As the virus buds from the cell, the viral protease cleaves Gag into several fragments, including the capsid protein (CA) that then assembles into the mature capsid shell (core), rendering the virus particle infectious. The CA portion of all retroviral Gag proteins folds into two separate domains, the N-terminal domain (CANTD) and C-terminal domain (CACTD). In mature lattices, CANTD interactions form only intra-hexamer and intra-pentamer interfaces, while CACTD interactions are also involved in formation of inter-hexamer and inter-pentamer interfaces. Our results show that, like lentiviruses, RSV is sensitive to IP6 in vitro and in cells, where in the mature CA lattice IP6 binds in a pore formed in the center of the CANTD hexamer.

For further analysis, we rigid-body fitted individual CA domains into the EM density maps of hexamer/pentamer unit pairs. These structures and models indeed confirmed that the mature polyhedron CA lattice consists of structurally different, intrinsically flexible CA hexamers that strongly deviate from regular sixfold symmetry. The hexamers that are adjacent to pentamers are deformed to allow bridging of the tube-like areas and the pentamer vertices. Further analysis of the different hexamers forming the mature CA lattice in polyhedral CLPs revealed that despite the deformability of the CA hexamer, local symmetries exist in the lattice. Aside from the C2-symmetric hexamers that are also observed in regular tubes (and are surrounded by only hexamers, Fig. 3b group V), a fraction of hexamers in the polyhedrons were surrounded by either two or three pentamers in a symmetrical manner and hence followed C2 symmetry and C3 symmetry, respectively. As the structure of the tube-like hexamer with C2 symmetry was already solved at high resolution from regular tubes, it was not further characterized. In contrast, the structures of the other two-symmetric hexamers highlight the structurally dominant influence of the pentamer, where it actively defines the conformation of its adjacent hexamers. Specifically, the two CA monomers facing a pentamer adopt an arrangement similar to those two CA monomers in the pentamer, causing an increased spatial separation between the CANTD’s of the hexamer.

>PVVIKTEGPAWTPLEPKLITRLADTVRTKGLRSPITMAEVEALMSSPLLPHDVTNLMRVILGPAPYALWMDAWGVQLQTVIAAATRDPRHPANGQGRGERTNLNRLKGLADGMVGNPQGQAALLRPGELVAITASALQAFREVARLAEPAGPWADIMQGPSESFVDFANRLIKAVEGSDLPPSARAPVIIDCFRQKSQPDIQQLIRTAPSTLTTPGEIIKYVLDRQKTA[6x]> MVFLPLKWSLATMSFLLSSLLALLTVSTPSWCQSTEASPKRSDGTPFPWNKIRLPEYVIPVHYDLLIHANLTTLTFWGTTKVEITASQPTSTIILHSHHLQISRATLRKGAGERLSEEPLQVLEHPRQEQIALLAPEPLLVGLPYTVVIHYAGNLSETFHGFYKSTYRTKEGELRILASTQFEPTAARMAFPCFDEPAFKASFSIKIRREPRHLAISNMPLVKSVTVAEGLIEDHFDVTVKMSTYLVAFIISDFESVSKITKSGVKVSVYAVPDKINQADYALDAAVTLLEFYEDYFSIPYPLPKQDLAAIPDFQSGAMENWGLTTYRESALLFDAEKSSASSKLGITMTVAHELAHQWFGNLVTMEWWNDLWLNEGFAKFMEFVSVSVTHPELKVGDYFFGKCFDAMEVDALNSSHPV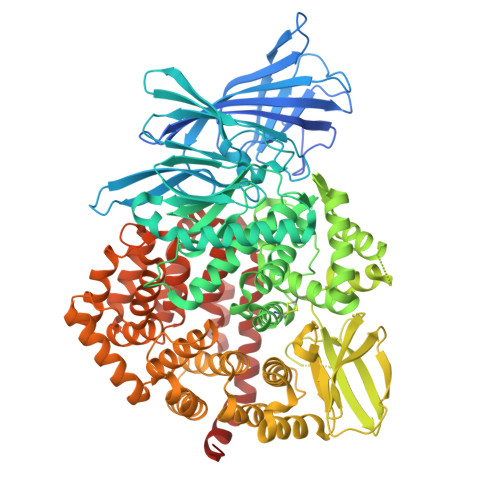STPVENPAQIREMFDDVSYDKGACILNMLREYLSADAFKSGIVQYLQKHSYKNTKNEDLWDSMASICPTDGVKGMDGFCSRSQHSSSSSHWHQEGVDVKTMMNTWTLQKGFPLITITVRGRNVHMKQEHYMKGSDGAPDTGYLWHVPLTFITSKSDMVHRFLLKTKTDVLILPEEVEWIKFNVGMNGYYIVHYEDDGWDSLTGLLKGTHTAVSSNDRASLINNAFQLVSIGKLSIEKALDLSLYLKHETEIMPVFQGLNELIPMYKLMEKRDMNEVETQFKAFLIRLLRDLIDKQTWTDEGSVSERMLRSQLLLLACVHNYQPCVQRAEGYFRKWKESNGNLSLPVDVTLAVFAVGAQSTEGWDFLYSKYQFSLSSTEKSQIEFALCRTQNKEKLQWLLDESFKGDKIKTQEFPQILTLIGRNPVGYPLAWQFLRKNWNKLVQKFELGSSSIAHMVMGTTNQFSTRTRLEEVKGFFSSLKENGSQLRCVQQTIETIEENIGWMDKNFDKIRVWLQSEKL>[4x]NRRYDSEFQTMLQHLQPTAENAYEYFTKIATSLFESGINWGRVVALLGFGYRLALHV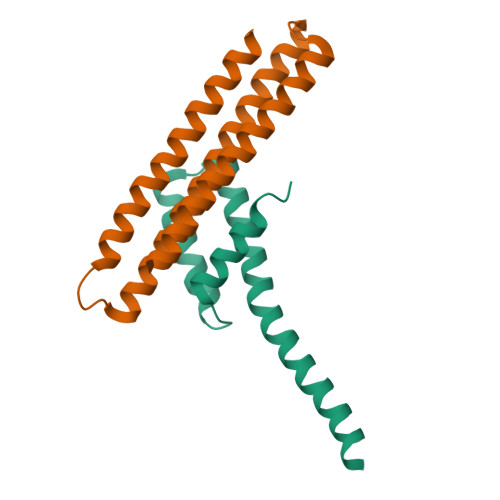YQHGLTGFLGQVTRFVVDFMLHHSIARWIAQRGGWVAALNLGNG;>[4x]GGADPKKVLDQAKDQMENVVRTLKQELEELAKEARKLDLTQSEKIELKLRYIVAHLAAIGDIEEAIREAKEEADKLKRAGLVNSQQFDEFKRRLEELHKEADRKRADYAEEFRNKLEYG4-[(5R)-5,6,7,8-tetrahydroimidazo[1,5-a]pyridin-5-yl]benzonitrile 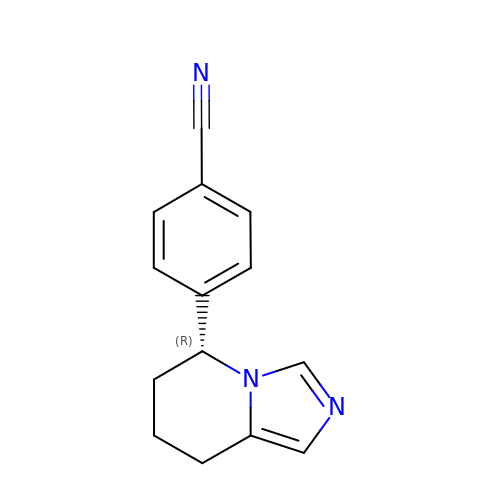| C14 H13 N3 | CLPFFLWZZBQMAO-CQSZACIVSA-N> MRDAVTTLIKNYDLTGRYLDRNAMDELKAYFESGSARIAAAAMINANSATIVKRAAAQLFEEIPELIRPSGNAYTTRRFSACLRDMDYYLRYASYALIAADNNVLDERVLQGLRETYNSLGVPIG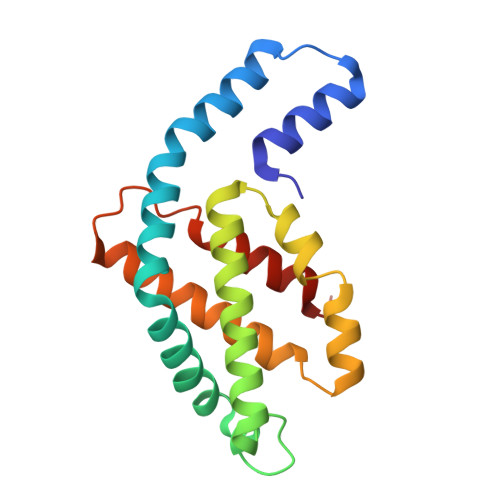PTVRGIQIMKEMIEAMAEDSSLNSTDFIASPFDHMTRELSELSV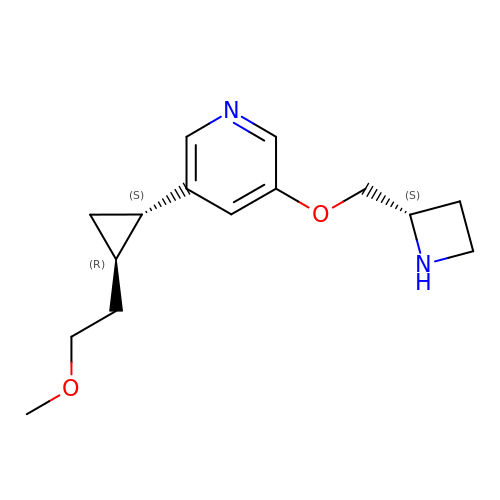3-[(2S)-azetidin-2-ylmethoxy]-5-[(1S,2R)-2-(2-methoxyethyl)cyclopropyl]pyridine | C15 H22 N2 O2 | NMIIKXFGCKOYRV-WHOFXGATSA-N(5R,6S,8S)-8-[3-(AMINOMETHYL)PHENYL]-6-HYDROXY-5-ISOPROPYL-3-OXO-1-PHENYL-2,7-DIOXA-4-AZA-6-PHOSPHANONAN-9-OIC 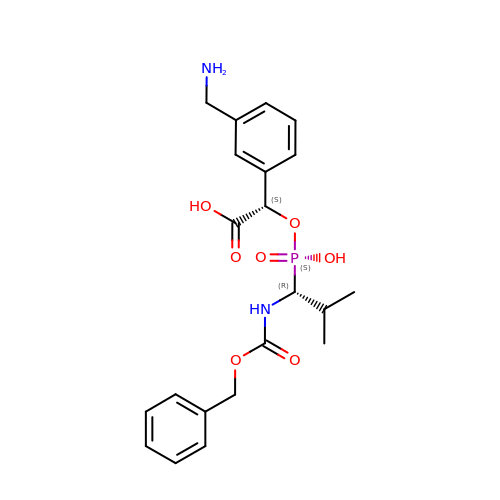ACID 6-OXIDE | C21 H27 N2 O7 P | RTFGEFWZCFCODU-RBUKOAKNSA-N>MGSLVNRKQLEKMANVRFRTQEDEYVAILDALEEYHNMSENTVVEKYLKLKDINSLTDIYIDTYKKSGRNKALKKFKEYLVTEVLELKNNNLTPVEKNLHFVWIGGQINDTAINYINQWKDVNSDYNVNVFYDSNAFLINTLKKTVVESAINDTLESFRENLNDPRFDYNKFFRKRMEIIYDKQKNFINYYKAQREENPELIIDDIVKTYLSNEYSKE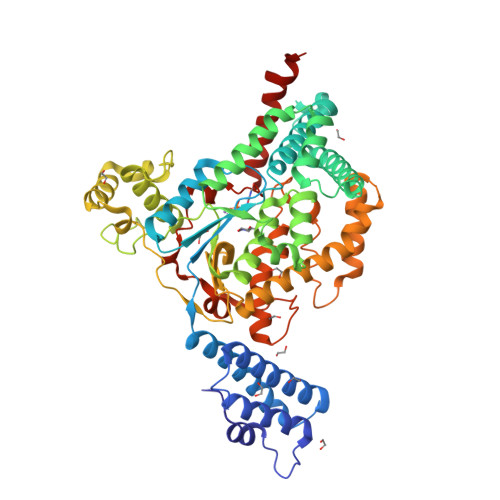IDELNTYIEESLNKITQNSGNDVRNFEEFKNGESFNLYEQELVERWNLAAASDILRISALKEIGGMYLDVDMLPGIQPDLFESIEKPSSVTVDFWEMTKLEAIMKYKEYIPEYTSEHFDMLDEEVQSSFESVLASKSDKSEIFSSLGDMEASPLEVKIAFNSKGIINQGLISVKDSYCSNLIVKQIENRYKILNNSLNPAISEDNDFNTTTNTFIDSIMAEANADNGRFMMELGKYLRVGFFPDVKTTINLSGPEAYAAAYQDLLMFKEGSMNIHLIEADLRNFEISKTNISQSTEQEMASLWSFDDARAKAQFEEYKRNYFEGSLLEHHHHHH[2x]> HHHHHHSSGRENLYFQGHMHNTLPTLILGAGPAAIQLAVDISATGDARLGLYNRPSTKGERLKQYLALTPTLYLQGTGKAQATQKESSVTIDCYIDQLAQAVGDWQRLILAVPADHYYAVLQQIPWAALPQLKSVILLSSSMGSGLMVQNLLNAAGKRDVEVISLSSYYADTKYIRAETQDISANTQDINAGTQDIGAIQPYRAYTKAFKQRIYLANQW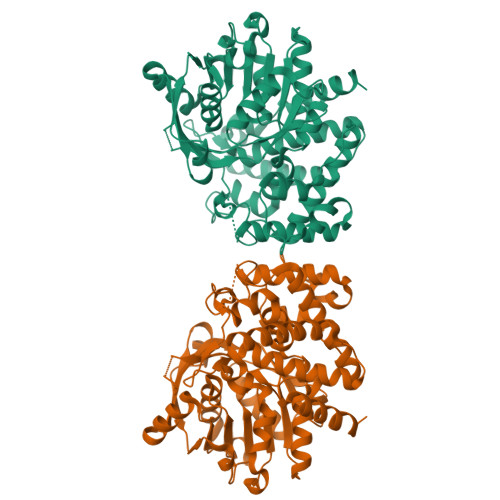GNAGSAEMSWLTAVLARHHIDTLPCSNLLAAERFSITNYVHPPLALADTTLQALFYPEQRSQYLYKTQPEGPVCPAVIADLAGLADDYKRLLNRLGVEEINLLRFLNDDNYPVPASMVSRRWIDEFPQLPPLEQQYALFVRYTALLVDPYSTPDEQGRFYDFSAVKVATVYQDANALWHLPRVPLEDVHKLRTLLLLAGALDVVMPTAQRLLQRFQQALKAFIDRVGEEHCHPSLLGDDCDRQAAIIEQQWRSQT>[2x]MDIHSHQQALDAYENVLEHLREKHIRITETRKAIISYMIQSTEHPSADKIYRDLQPNFPNMSLATV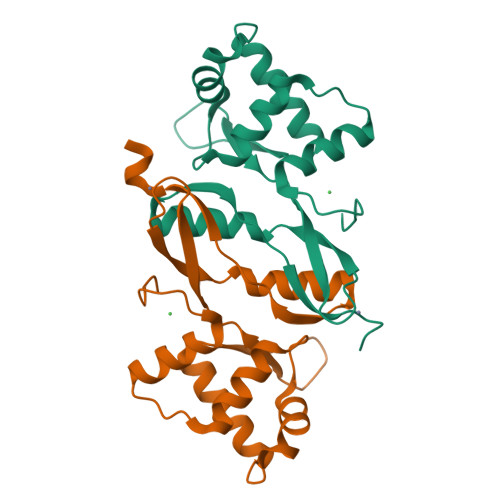YNNLKVLVDEGFVSELKISNDLTTYYDFMGHQHVNVVCEICGKIADFMDVDVMDIAKEAHEQTGYKVTRIPVIAYGICPDCQAKDQPDFLEHHHHHH>[2x]GHMKISRETLHQLIENKLCQAGLKREHAATVAEVLVYADARGIHSHGAVRVEYYAERISKGGTNREPEFRLEETGPCSAILHADNAAGQVAAKMGMEHAIKTAQQNGVAVVGISRMGHSGAISYFVQ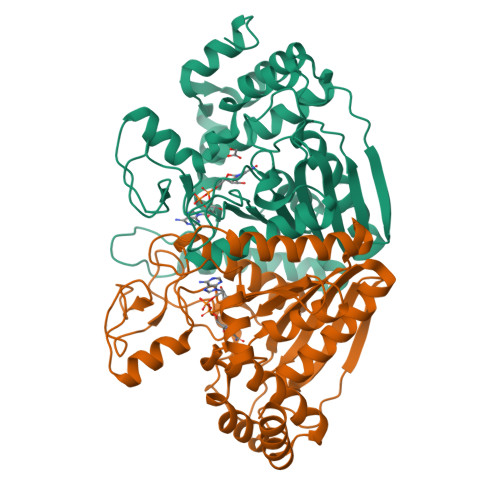QAARAGFIGISMCQSDPMVVPFGGAEIYYGTNPLAFAAPGEGDEILTFDMATTVQAWGKVLDARSRNMSIPDTWAVDKNGVPTTDPFAVHALLPAAGPKGYGLMMMIDVLSGVLLGLPFGRQVSSMYDDLHAGRNLGQLHIVINPNFFSSSELFRQHLSQTMRELNAITPAPGFNQVYYPGQDQDIKQRKAAVEGIEIVDDIYQYLISDALYNTSYETKNPFAQ>[2x]SVKLAGNSSLCPVSGWAIYSKDNSVRIGSKGDVFVIREPFISCSPLECRTFFLTQGALLNDKHSNGTIKDRSPYRTLMSCPIGEVPSPYNSRFESVAWSASACHDGINWLTIGISGPDNGAVAVLKYNGIITDTIKSWRNNVLRTQESECACVNGSCFTVMTD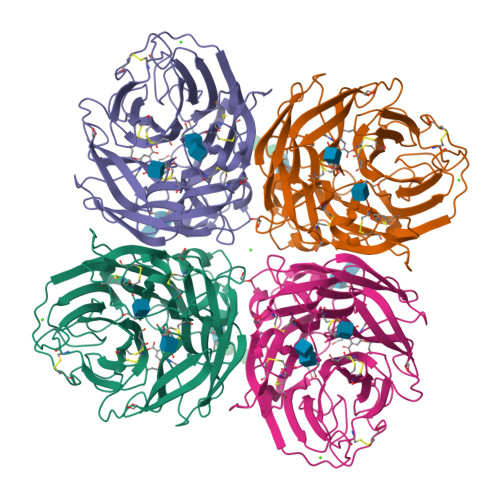GPSNGQASYKIFRIEKGKIVKSVEMNAPNYHYEECSCYPDSSEITCVCRDNWHGSNRPWVSFNQNLEYQIGYICSGIFGDNPRPNDKTGSCGPVSSNGANGVKGFSFKYGNGVWIGRTKSISSRNGFEMIWDPNGWTGTDNNFSIKQDIVGINEWSGYSGSFVQHPELTGLDCIRPCFWVELIRGRPKENTIWTSGSSISFCGVNSDTVGWSWPDGAELPFTIDK>GSHMARIDARLKEINEKKILQANEVLEHLTRIALGQEKEQVLMGIGKGAETKTHVEVSAKDRIK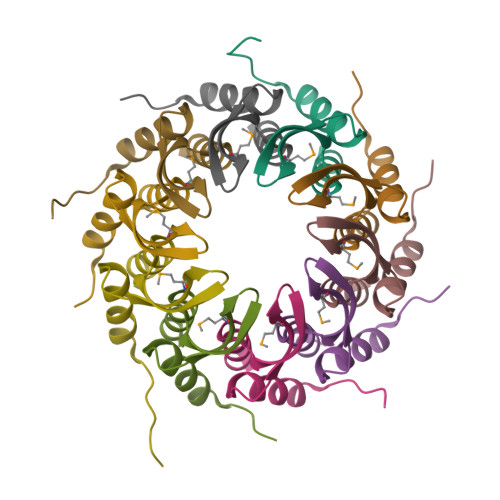ALELLGKA[10x]> DVDECALGANPCEHAGKCLNTLGSFECQCLQGYTGPRCEIDVNECISNPCQNDATCLDQIG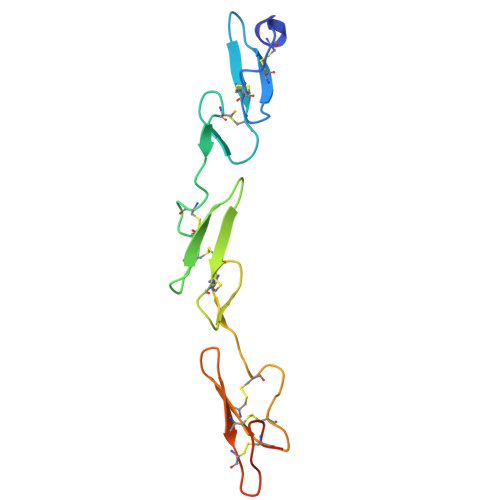EFQCICMPGYEGVYCEINTDECASSPCLHNGRCVDKINEFLCQCPKGFSGHLCQSGRLEVLFQ>[2x]GSHMIEIQASQRAYILEEMAVQLKKKAEERFSHDEYKVGRIKLTAGEKVDSEEDIKTISVYMAPSSEKTVQTVAPVHIDTDHAYVTKEAAEQKEAKQIQTQLADIWEIGSEKITVHMEG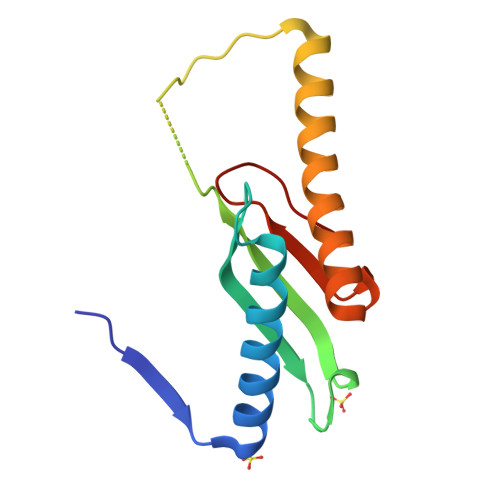GESVGNE> MRTTKFLALALCLLASASALSANNSAPSNDWWDIPYPSQFDVKSLKTQSFISVKGNKFIDDKGKTFTFRGVNIADTGKLLSRNQWQKSLFEELANNWGVNTIRLPIHPVSWRKLGPDVYLGHIDEAVRWANDLGIYLILDWHSIGYLPTEQYQHPMYDTTIKETRDFWRRITFRYQNVPTVAVYELFNEPTTMGNTLGERNWAEWKTLNESLIDMIYASDKTVIPLVAGFNWAYDLSPIKKAPIEREGIAYAAHPYPQKAKPEVKNDKNFFKLWDEKWGFAA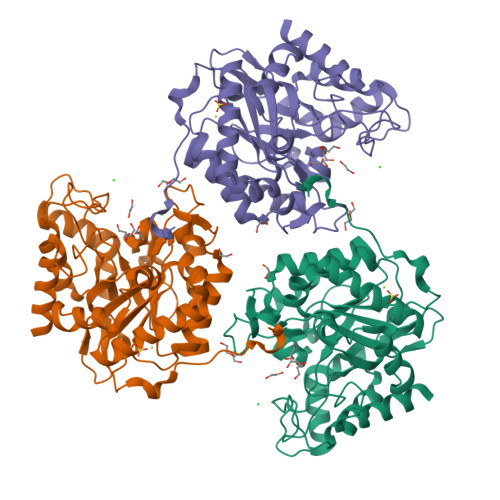DTYPVIATELGWVQPDGYGAHIPVKDDGSYGPRIVKYMQKKGVSYTVWVFDPDWSPTMINDWDFTPSEQGAFFKQVMLEAKKR> GVPTYLLPGSGQFLTTDDHSSAPVLPCFNPTPEMHIPGQVRNMLEVVQVESMMEINNTESAVGMERLKVDISALTDVDQLLFNIPLDIQLDGPLRNTLVGNISRYYTHWSGSLEMTFMFCGSFMATGKLILCYTPPGGSCPTTRETAMLGTHIVWDFGLQSSITLIIPWISGSHYRMFNNDAKSTNANVGYVTCFMQTNLIVPSESSDTCSL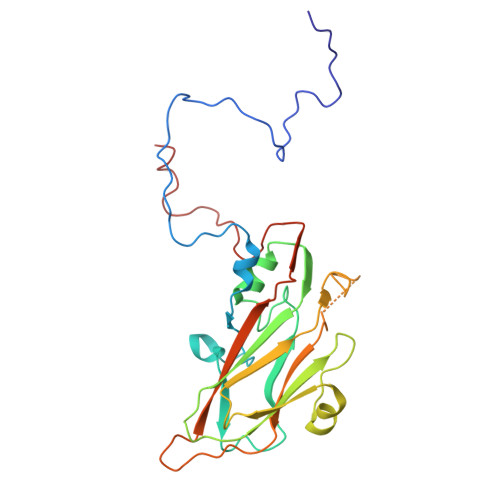IGFIAAKDDFSLRLMRDSPDIGQIDHLHGAEAAYQ>[2x]MAHHHHHHMTALKNDRFLRALLKQPVDVTPVWMMRQAGRYLPEYRATRAKAGDFMSLCMNPELACEVTLQPLDRYPQLDAAILFSDILTIPDAMGQGLYFETGEGPRFRKVVSSLADIEALPVPDPEQDLGYVMDAVRTIRRELNGRVPLIGFSGSPWTLATYMVEGGSSKDFRKSKAMLYDNPKAMHALLDKLAQSVTSYL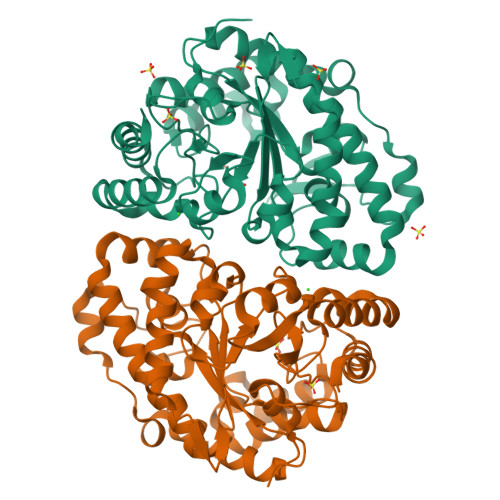NGQIHAGAQAVQIFDSWGGSLSAAAYQEFSLAYMRKIVDGLIREHDGRRVPVILFTKGGGLWLESMAEVGAEALGLDWTCDIGSARARVGERVALQGNMDPSVLYANPAAIRAEVARILAAYGKGTGHVFNLGHGITPEVDPAHAGAFFEAVHELSAQYHG>MGGSTKLEEHLEGIVNIFHQYSVRKGHFDTLSKGELKQLLTKELANTIKNIKDKAVIDEIFQGLDANQDE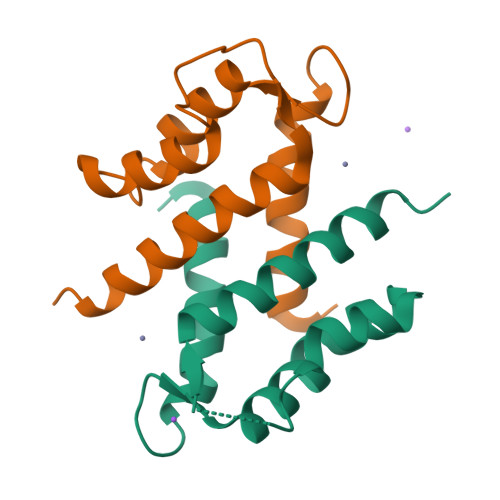QVDFQEFISLVAIALKAAHYHTHKE[4x]>EAEAEFLGSTCSSPLTHGSAAPGDPFWLQNIQHQGIAAFNGNPGGYPVFRNVKNYGAKGDGNTDDTAAIQAAINAGGRCGQGCDSTTTQPALVYFPPGTYKVSSPLVVLYQTQLIGDAKNLPTLLAAPNFSGIALIDADPYLAGGAQYYVNQNNFFRSVRNFVIDLRQVSGSATGIHWQVSQATSLINIVFQMSTAAGNQHQGIFMENGSGGFLGDLVFNGGNIGATFGNQQFTVRNLTFNNANTAINAIWNWGWTFQRITINNCQVGFDLTQGGTSNTGAQGVGAEAIIDAVVTNTQTFVRWSGASSGHLQGSLVLNNIQLTNVPVAVGVKGGPTVLAGGTTTINSWAQGNVYHGTNGNPTFTQGNIANINRPGVLLDSTGRIVSKSHPQYTGYAPSDFVSVRSQGAKGDGHTDDTQAIKNVFAKYAGCKIIFFDAGTYIVTDTIQIPAGTQIVGEVWSVIMGTGSKFTDYNNPQPVIQVGAPGSSGVVEITDMIFTTRGPAAGAIIVEWNVHDPSGQQAAAGAWDTHLIIGGTAQSGLQVGQCPTSGAGGNNCFADFLGLHLTSGSSAYLEGMWVWLADHDLDSGGSQQISLWSNGGIMSESQGPVWLIGTASEHHINYQYFLKNAANHYIGLAQT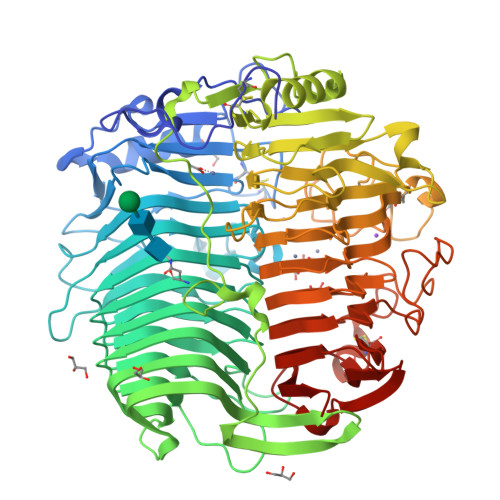ETPYFQPNPNPPAPFITNSNFDPSQLGQGDAWAMTVQNSHGILVFGAGFYSFFSAYNTGCQSPQNCQNQIVNVDSSSDIAFYSLTTVDTTWQFSVNAQGVINRSNNPNGFADTITAWTRN[2x]> TVFRQENVD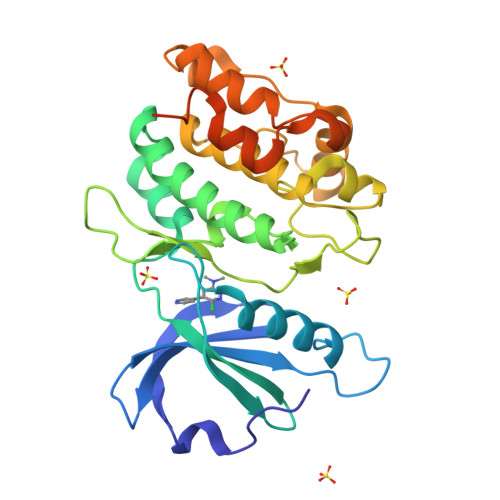DYYDTGEELGSGQFAVVKKCREKSTGLQYAAKFIKKRRTKSSRRGVSREDIEREVSILKEIQHPNVITLHEVYENKTDVILILELVAGGELFDFLAEKESLTEEEATEFLKQILNGVYYLHSLQIAHFDLKPENIMLLDRNVPKPRIKIIDFGLAHKIDFGNEFKNIFGTPEFVAPEIVNYEPLGLEADMWSIGVITYILLSGASPFLGDTKQETLANVSAVNYEFEDEYFSNTSALAKDFIRRLLVKDPKKRMTIQDSLQHPWIKPKDTQQALSSAWSHPQFEKSAWSHPQFEK> MFLIHFVHYKTILQKYTFKFKHIFLSIDKYNSLFFNISGILIWLNIIHINIILIKYSFFILINNFEYLIILIST;> MFRLTAASQKNLNSWYTKGTMRGGVPRIYYAWMRPGSFTRRRFEKMRNPFVDLETGTSLYFRDTRDSAEAIAHAADSKGIKGMDNAIDLYNEYRIVPDLYPEGFQWKHKLNTEYNQWRSNTWLTPDLIPKEHRGRFLCNFQLNIVAYDMRVVKFSPKDHRQWIYCVLYVGSGKGIAGWGRAVAPSTQEAKKEAIREAFSNIIAVDLEQEGPMYPVRVNADGVRVLLYPARRIVANFRVADILCAFGFQHAGCRINLKATNNPKSPTHTVEGVFEAVKALRSVSEIAASRGKVPHSLIYNIYPYLEEIRRRKGMMAMHPPGKDGLLMPDRVVDNRLPDHLKRGYYDDVYWKDFFAGSDEHLNEPRMGLRGDEMRRRLEEAQTSPAPTTAKDTRRRTLEDVLKRLGKTTRDLGSIPIVNPRVDVGLPTHIKRNYQLH;> MVFYSFVLVMKPRQRRFTSQALREIGVAVYSNGGLIRSITNEGIMRPYSRFRDADNTPLTYARYIILQLDMGEEEMGKVDKIIREHQDVLMALKLNNLERPVGIRSGNKELQAAYFPLDTFTRLEEEINWSPQTSADIYTQLEMNWKEFSRTRWSSFLRN;> MLRQSLLSLAKVYGAVPPLGAAQGHRLLHGKREREGSLFAVANDVKRDERLLRQQLNALLEEERMPMQARLQRNEAVSSHEAVPQTPLVDLPGVERRRDLPADPITRLFFQHKGDHALYYGTYDKPSVQDDDRVQIEKRVPRRREENLYTPIYDFCHRIREATEQRKRFVVVPSTIETRGCARVMHDHGLVAGFRDFHNDRAFAVELKYFQGDSTINVIEPCSYDGRTEFEWSPKMMRRLLNTHGIHNRLVVYICRTADNRIIDHIHAVKENIGGRGLMMVH;> MQKLLSPRTARHARLFRLAGKLADSGSPGVPKSDGERLVWVNSHVRRDKDISLSQEEERIRELMMPLEVGENSFAANGQATHGNLFYFREYPMYPGEYVPAEHNTLSSLRDELRLDLTAQSLKEAWMRVSGGVYFQSVDEYYASVDGLDAEQIGEVLAALFPELNCYEAQALVQRTLECISRPVSAASRQLSRTITAEAVGLDNAPGHYTNFLEWMGRLTETRAFKTEHALFEFSRRKFNRDDVRVMFENYRLMSKATLLADSADSYSHFYTVLKDFARKVAGEDSRHQIGVRIDEAEVDPETGIAVGRGCADGEKYHFTALLRENRDHNGIITVMGKPLSLVLDNKAWLMEMVLMPFDEANLDYRDFDAHIVSEGHAMPSIANEIAAFALRMAVANALVKLIPLTRIPLKKSGLLSVDRRRERGQFPGYLDGKKVKRRFAKR;> MVRRSHVVAYYWSRYRMPTQMPKFDGPAPVAAPQSMNSTKTNEFIDPIDDKFPMSIRGPLVRPDVPEDQYVDSWYICTSMTHHMGDYRPWSASAPPNAFRFRPFNEFDAKGREYVQYMREFARFDPRKSRGNGQKGFPFRDAYLTKMNEANQKTPPPTLETIMDRAVREHHQHARILSPLEVQRDVGRLEPIPSYAGKINADRSVFPFQWKTEDWYEYEVAKVRNRRFVFENTEEDGIRGSEVTYKIVLEGFWDHHVMKLAEDVCMFLKDVGRQIVEEKLVAVRRLLQGGAVDPELLAAFNCARAGPFGGLDEYDKEEVANFLRSDLRRLEEQCLSVINRCNVPVPGATNIYDPHTSWPHVEKLEPWVRMAEFWTSSSDTSFTELEMSTAHYEFRKFFRVIICKLPFQSTEFEKRMYDIRHWLHRQTSCEFHTIYRRNVIHDSAVFPTEHDPATPTTHEHHRMFSFALDWQSAPVNRLSTDTVHEGESWDAVAQRLGCSVGELKDANAERETIEAGVVINVPVTATRRLTSFGATPLVLPLKTTSAKDGERIRTWEEAAAILDCTVEELQQCNGHAALTYQKKESEAGEFDSSVTELVAPLSCWTSTSESEFSPVERVHANDTLVAIARRLQCSEEALRAVNDGITDVSGLDFVRVPPEARRPRRLVEPQLRPQAATDALLARTIAEEETFKLKSIPHLPQNAERFPHEYHTPTSRFPPTPSETPATQDWMAYTAKYLDKQFTISAEPAPVYNVNKLWPMQQIPGKVDQTPFEEDQTWLLHSIPVQQLEMHHHEKDLQDLPFINHEQFPRSLEWNAP;> MMRKSVTFLRRGKPRPRAGMFPDKYRRVPMLLKPQQGGQQYFNHFLIRSTNDRLTQQDVDNASGQAHSFISPQLPQMDWRNMSARSSEESIREEMRQLAENDVMQHQRVFNERMWYEKEEEHRMKARSCPEETSEHAISNDGAVPPPRVLGGDYFKTRFGYSLVKNSEMTQGPVDYSQLDMWGEMPRYTSDMVFLYLVSRRRNTYAVAYTYEGKRILNTYTAGNRGLKGGDRGFRSEGSTDNGHQVTSMYLNDLLPKLREMRASEGRPMGRGEKVELVVRVMGFYNGRQGAVRAVQDRANEFHVRYFEDITPFPLNGPKMPRGVFK;> MFCFSRGLWMRHIGQDVPKRHTHFVLESRLMYEKSFRDCWLHSVCRAISQLDEPLSKTVVGTHQKMLQRKVTCFQYNQYGLFKTPYYRLANVDRYHAVQGVAGTREWVPYVNVSYWTMNKMVRGGNLLVHRVHYTGWGTDSHLKKGGWEHRWNKVLQRNVLQYSRI;> MFVRSFCFLRKYGSKSKTPDLKTSFTKTTNFRKAEKISITTTDGEIVKGRGKIRRRTHSALKEAIGAMEHPAIWLWYPWRMNPEPPTPHMPQRRALKNVHGAVFNDLTPVQKKRQEQMLYGVNIPETRQMKFEEQHPLLAGALRKLEGQPKGFPFWYRKYPTRRHAYEYRFSIPVEMLDGYNDDVKKALSKGMMSIQEKQFAQEAMYMERYAEHDFDTTSPAVLAVKRALKCRVLRNHLLTNPHNNIIKTVLANTERKLNHALRRLRKVDFKKYWEIIRDHDVQDILQPPNLVTYRQGSYWKYDWNAGLAISTNLADVMDPRGLNGCVETGRSRSEVARDLGLSYTRPLHENEKKQLSHQAVYYERLAKFKMEQPEAARAMERERFVRKFSGMFVKMDIRSGAPDFPSTYRRLLGTKVVRWASKRHGPN;> MQVTETVLARAVIKRRSPQLWGAPGAPIIRMRGHHVVWKFQSYDLVVEHTHKRRNSDIRLLHYLGKHCPHPQKSLWSPDTPVAQDRHLFMLTTVDIDAFKYWFGVKRCRLSMKPWALLAKAGLLPPSLTQNSKIMPKPLFDKESLMRYYLANRKDEDVMAREKYLNYENSMVKTEEERAAERPVAPYL;> MLRRSLLAFPWWNFQTEHRQRCVLMYGGARTKNTHNANHRVFIKKYKRNAFPNRTRHHWAVSMTGVLSQRPRRMPWPYDLTSLIFNQPRQGSDKIGYVVGTSMLKTAVVATNHMVYYPKFNQRVSRTKRFFAHDEDLACVEGDLVHIKQCRKISKYKHYYVFSILEPNVEGRERLKLGLKAVPPPLFGYPVSRRIVKLNLTSTEGTQEKLAAAIQEHVQDAYRFSGPTPDQPRNRLADPVTFEDANNMIAPNAPAAAALDASDSPPLLDRGEYTEVEQDTRNKKGDDYWMNLQPKEKYDFKSFKKSPRPLEDQVDPRLIDGKYDIPTTASENLYFQ;> MNRTGGSIYAHALSQFAVCRQPWNEYIGLLTKQDSTPYHTEPQEKPAYRGRKQGREGWLFGQQVQLHYHRFPDEQLITNLSRWRTGETVGDIAMQQFRNAQPFDIEDKDPQGVQRPSPEVYMKLNYKNPATISRFLTRTGHMYPADILPLNPEAVVKLRVAKAQAIRIGLYPRFGNPFWFRSQKFRPKAYQENYDPTTYSTKRTVEHFAYNWVQTDRIRRYFRELEAVHTSGSASARGSGGGTTAEHKQQDQFYSPENQPISLHRNNISYMEDVGRSVKNPTVPGLMSTKGMKKKFHNLYSSTSTKRMGFSNPTLGIKKV;> MAFRNTFTTPGKFSTVSKNIVLLLIWRVKVFLRAEGFAHSLVMLPVSLYSKILLCDVKKKIVYFHCCTRKKSMLRRCPCVWPDGPTKSSVSIGTAFTLQKRFLKIAKSAFGFYLARRGQRKYPFLRRPHIKNTHSMNPSAPYFWSFMTAKSQMAFLPEENYITGDWTGKFFVSKRQVYTLQHATSGAKVRVKSFPSIFEFNSPSRWNIGKEMNTLTKPRMDLIDEQMLTKKQRLDYVRAGLLPK;> MLRRAYIQRRYPFNKRGPREHKSWKHHVLTEPPKPLQWRDPKVWTRDLSVMKSFDAPQWDLWQSRPRSEDMDEALQPFMDMPKSLKDRRYDIPWWANPFGAWYLQNILSLELLKLKSKTNAEKIATYRSYMRSLASGKDNTMSDDDVIRNIIKERWKTLEFGDRNAGYPCTFGDYIQFLNEWFKSLDEEGMQRLREHFDRRIRPLLAVMSPVDILWLEALTQNSPHNKEQLQRKIAFQTSLGTPEFFDMSKRLRYEINEDYKVRDELGPELFALWSKAPERWPPERLSKMYGLDFTLVRKILVWHHFKACYDACVEPDWSLPKRLFALEWIRDVRARKHGLFYGKMRFAEQKITFYSDRFLFRDLVNRREASYANVWEMDDPYRFLQTEQDYEDYWGDNYDVYRRMFPEMIGRTGEPVQQYGQMPIWAGPHRQHANKSEHNWMFAEIGVNVGHEALKKLELDPTNEKRRRFVIRQPDGTLRSAKMSEMRAWYWKEEWADFRFWAPQMEWGIENTPSQEQYQEHVPDTTDADFRKQRRIQSRPVKWFYESHYTRTGSFAGFQPLRFMQRRTEREVRWPDVINAAVQIQKRKPAAYIFKAIPEL;> MRQCVVRRYKMPKNMGVAPRFDTWNEKYEPWEHMKRMGRLVGTGFYIPPEWYNHFRMFPPINHNFQQEKTLNPHNASEPTQDDTSTLSPERVALRDELARKSRLVASEGMRYYNIFWVRKPLDTMEKEYYELKRRGVDHGEAIRKVLQGFYSGLAVKKRVAAIQAEEAKLTGRFITMREATVVLGVLAKLHKEQLTPHQVSLLAKEQGETTQSGAKLTAIVSRTQPHVNKEASSPATSEAVGSSTEESLSADALASMLSEDGEQSAVGTRYQVEVKETANDSVRQLREKAEDQTGFPDWYTGESPTYSGTS;> MMRSSSFCRRQIRPYYNLPSKSEHGRKMTGFLTPYRHWMWKQNELWRNVHEAQFEHLRRVYKRQWLESFRVNADEYIYKYNITKAAQLAQWECEMKEQEKKRIEARQMMDGRQALKKKHLDLLREFHERQFFFWYERASERLQNMNLINYVPHAQLREHIDKELDKYVAGKNEPYPLNFVGQMPFLEDGDGNIVEVPESLLSNHMAEHPDSTAKPHEPHTSSSISEAAAFEERMLRAMVSAKEEDLKEWLGDDSRALSETIDDISREEEEREADIRVARSMEETDAEREVSRRAYIERGKTGSRSIFRPPTVSEGAGGTPSAPAGDANTPMRRRKKGKLDRVHALQAHQDELLAKLSSQGLKEGVDASSVPERGKIVQSRGRIRDKAVIPTHEVLMQKPELAAGSTPGARIQTKDMVDKMYHRGKYKKSGSGDKSDGEDL;> MRSKTLKKSLAAMYMRPPVTCYTDACEAPVAMWDGAIPLKETRKLKNGVPVRTVSRTYSHPPQLTPTQLSFNDINSMYCVGNDELIQFFPEGLGGRVFQTMPPGHPRGFLYRKETHLLNLFVDKVQHWHTKRSVLSSLTNGRTGFIVDGPTGCGKSALMCQVVHFARSRNIVTLYVPDAKVWTHGEWCWPSTILPGFFDAPDAARSFLKYFAVANRATLTSWKLRCTPKDLPTEQGERQPQNLYELCEWGHRAVAPASIDRQSVCVKFLMDELSEEKKLPVVIVVDGWNLFSHETHFRYPHPDFLRGLASFNESSTDIDLYPQELPRIPASRLSFVRGLNKMILSGDDPNKFFITCTTRDFKPFDGISGFPNVETDRFANSLDEYAPYDPEKDSHFHPIQIGNFDEYEYRSFLRFLINSGELAGLGWGPLWHASSDFERKLYKIGFLSGRNPQGVVDHYHQELVWRYDYQRTRQKQYLLKRRMEGMSRGASSGAVGVR;> MVLRRWFPLLGVHRVGYTHPSTLPVPCAQRWDLRLARARIFQEYIEEKAPGAWQLEDERSMSPEFKTFTGYPMRDMRPGYGQNLPDYIMKKRLPNNTHYELFARRDIPNEDNAMYGKYLYDMTVHGTSLPSTYRMHKDINKAQRNDRKLSGNRFKVLCSSGAKNPPSGWEPIPDATEEEED;> MLRCARVALRADPLNGGSSMTLGSKGSKLSPEPHRRRMPWTAAKEYVPGVVLNARDKMVLDGVQLLDIESIDRASQLDPLEVLRAVVATREYNISTGKNIFQLASQATYNGRGQRFYRKEWQEGTYDKYVTLSAIDFDRDGNKGTAYGYITFHGETTTRPVQVDFADVPGWYMDFVEERAVPFTGIVPPPPSIGTDVPVDPHSYRLKAYPYYDAPNPPEFVERLLKDRGVLPDTPTETADVDKDPTTSDGSVHYDGK;> MRRWHRSLNPALFGERGSGHYFSTTRARLQLQAQDRIICGTHGAGIVAHQTAVNSSDNPMLSSVTTAAPAADLSRTKPHEGTGTSERDPYIRTLHNQRSAAPESSVSQSHTVNAPTVDECEMLAERWGTMNYWHNDTFPRLVVFLKKLLVPDVSPLSPTAESLLSMFEKVVIPKLTSDEEDRRKLVSLWSETTLQAEAAVTKFLFQRGSFESMLHRIITDALEKMSTLALGGQEGNLALEALKRQTLFKRNDYIQKRLIDVVSNSAYLGYGDSVWQVFFAAVEANEENLLSDRATTDAIRAAWEGVMREDVVRLPDVTGVVALYLTLVCIRESGRLVPEELKELSSGLEDGVRPGVRKLQQYPLIFLHPTVKRRFVVKAVAEILHNSSSNAFSNMLRENGLHDTAREVALCEAMNRNKELAEGDVGDAVGRFVSKGEVKTLLSSLVSGTDAVVRDAVAGIFGIGTTITIDWDAVMQNVDWSNNWQRLATALLSNSAVLSAIVKLVKNAIGAKGMSKHLFTDEYADQLQLILDAREERAASRKQRIENIAQELSSFERVDLSCDLLRKLGVDMTELDTAAAATRNMNVVQRPCIEDGLLSLVLEAVTKRHPNWVKAGVIQTTLKDPFDALRWMMHIFIRLSYVPHAGAATIARLSRRRIGPIGLEPHQFNVPAELGFVEQYDNLQYKRYDWQGWYQRMLDVHNRNVSLRCRICDLQRLDGNGVQFVDMQTERRLRILAQHRVGMGVLKLDADKYEDQADNVTFGTTKLSELLADARKAQLGEEYWPSVELKVRKPSGQSKAHYSLIDNERIEKRSRELYEKYRDAKKRSLFVTPMETWLEVKGMQVRKSVDNADEDGYTLDALQDMMDGDDGDKV;> MRAGCVACSRIPKLGIAALGSTTTSMQATCQETQELRCATTQMAPAVIFPLPPPLRGSYIDRKPTAASFNEHHATASFRHHMIASADVSHRPRHFYFASGTRNDTGTRSVKEGERKQLKQQTNVEVDSVAYGDQLDELSARWAAKFYGQVTFGPRNYPYPSSRWLARRFQMKKHRIIKRFRFRRYKLAAVANLPFAKMIRVGMLPELKSSKTKRGDVVDPTLSGQLVSAVKNTGEKRKGQRTRPKSKYQV;> MLKRTLTVLDQTYGPHKSYKYTYMPDPRKLAPIETTQRSEIVPQSIRPPTSYVPNHETFLERADIHRLRPTSDFKASFKDWNDLFTCDKRQLRVRGIPRMTRDAIRTAVQAFQNGNPPERFDTKEEWLYYKQFKTVDYSYRVIPELPEKYRPHQSGIDQAPLPDYREINKMPQWAECEERRQSKKTV;> MIRRRVCDGARLAPNIRATFSAVRYQSGLHTFIRDSKPSNFSSVRRSENANGDATASPGATAGENPASSGDWASHMQRELFGEVD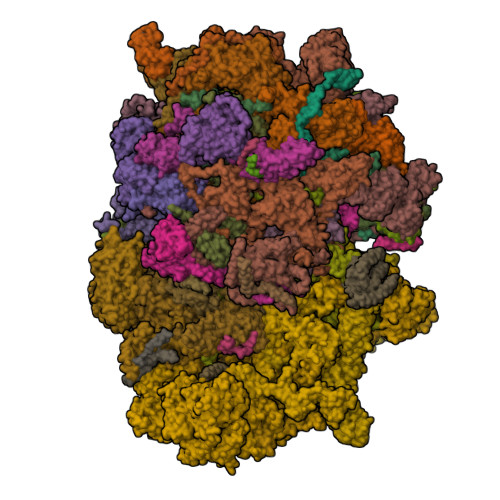PLGGQAHKDYYRDVTRGYSPQYAPRNFANGGAVAYPHIQSPYEYEEAAHRRVWLDHDVDRMREEFTQHRASLRSLASAQEREELLRSRAAEYQVANTVHESESVHPIQQLYNSGGTSRSALKQQAVADRYSIAEQHSPLPLTTGVDRDALDEAQRTKDRILNDSFTAENLLITHGLREKEKHDFTILQRTVRIPFQGYDMDRFLAQQKGTPYGAQQLPPNVVPSSMEEAQRTLRGSSATATPLVDAVAQKVYARNTVVDRPAIGEQLTEQIINIMRASRTTAEQQREEERAQRFGLGRQGALVQDGGPDQRTLKKHTNDERIVDAMLFQQNAYRKTPTDEHWNPYIRRSTENGVGHLLQNKFDIMRREDRLSKGEQDLTERNTIHYGVPIQQIVDEFVFRHRNARGERPLDYFKPFPNFRALRLNRMYRDVEGFSLMKQRPEFLEWELFTRYRQHHQQRRRLALLHGLEPVANETAQERDTRRHRLDEICERTPFDEREMRVNDDEMRVSVETLRSWFGVYMLPSPTVVNAVLGGSASVNLHLYHLADEMGTADTREHVLSSRYLNRLLLLESYQNRVGRGFMNHVVGRAPEPVVPHEQPQEVLRHFSAEERAMYEQHVKEQTSRQLGEWERAMKRRRWLTDHQQYGHVVSHGLETSVVDLSHTETGAVLTVSTKAYEQEIEAVRMKTNATIKVDGMVYNLLPNSERRVVPLTVQLDSGEKIDMTSEDFDRCELEAFPRNLNHALNYGIANYAYNRGNYVETQDSIWEEQTASGQEGWSPATHADGLREGLPVRARRPIFSSSAEQRIAGGPQRAVIIQYHHQPFFNPEPRLVKVAFQCDGTIMEVPISDVMIWQRRYHGPERTVGDESRRYNPAAMRRYVDVTDPFNEKTSNTEHFLDKYEPKRNADTVADKYRTTKQITEIDKWTRYDSARADNYRPLSISHRRDYIRMGYIPRYTPWEWIAIQEADQPLIAEQIRQDNIGTSYFFSLNRYWRYKASPHGYIRHFENEVRDLLQYVDGVTPWKQAQKIRTYWEVRSHHPMPQFNRPEVAMHRNTVGLLPAHMWETDKKTGKVKSVKDSVRDYQTKTPYPKWVQL;> MFRVRRLAGFIQCSPCGKMGPLKQQTRRYTPIWKSDPAVDNVAPLRDEDERRALWAEVGPISDVGSAVTAWIRFGNDPVLHTAVPTMLGGKFRNQQREKESLLPNSSSPFAYVEDYMGTNLVFGSPVHAKESAAVWATYFERRYASRLRLSRRTVANYVGLINSPEVFDDESDRPETRWSQDTFFRECAYLSEKFLKEKVSNMQQFEAALKRASPEAYLAFFDAFQQQTQTQIPLPSPSVWHYEGERRKQWAEKFISISHKAQAFFKDVLSEDVKKYQEVPGKLLQKVKPVLADVGKILVKRHERWLKGRVWTSLTEEEREAYCMKEVKRQQMQVEDGEFDPMMEDDVDDTELEEWQREHDAIMKLMNSPIDGLHFTTLELWLHTMRCEELETEHIYTSARVRAIQVAARKKLYDTTSYEEVIQAVVESIARGTLDLGAGVLRPHFNEVWCQLNYAKFGSSTITQHTTTSRRQLLFFHAGSLKDIAATATLYYATKPLSNSLDYASPYKYRRSLITLCSNYGVETAYTTQRPLLRSAANLARAEDLIHAVVTAAAQPFGERRRAATRDLHMEFQRLAVPVERVIVANPVSALLESGADPDEKPVEGEKVNMWPLGAKRVVLYKWSAPNVEKLKAMESDAASAVSGSSLTAKRLREIQELKRRGFLEVSLWRRVTAQERKQRNEIVEAKKKQVEEVVRTVPSLAHLHQYATSLYSRIEERVAFPTETSTVTETTNMKEETNKPLEDSEWEFAVLLDDRVLLNKEESVELYLPYRDANGELLAQGEYRALVRAFDLEANPNLHPAYCSVGYSESFQVFDALPQLIAQFFRVKDATAEAAGVTHIPAADFTPFCAFLRDAGLDVPLRCEFEAGQAVTTDGDVYMDYFLQLLRGEAFHQSHAQAGLTEAQRAIEPLCRAHWVVHHPGADESEWATARRSVLDHAMQHEREWWFPNEMLDVKDVVTGSTNGLTPQMYPAAVRYGVELCTVLTAEGKFVDERGSGLSARCVVNGTGAAESVVFDTANCNGTNTTSVEDALRVAHGALRSAQDRHNTLAAFRLGPLSKQSQVLLFCGVNAYEFGGKYARTYAYAFEKAKKELEATAASGFMAPSLSHEDTERLSDQPTTSPSVDRFASTTHPEQRKAQFVPRVGPGSTPLEDPAADQKSEWS;> MLRCTVVGHHRSGKARAFVFRDPSLRMMRAGSGYQQLRRMGMPMQVGMGWRKVDSFHANTQYQHAWPLLSHDDLGNSDQSNNTKNIMYSMYMPKRNKGTAPWFRGADTYSVKYCEQGRYEYQRYLMINRFPSEYKKHFLSFLSNIRMSSGSATIPQEALHWLLRMIVDNFNPQHVHYIAAMKTLQSAGELDMARDVWKIMERQQTWPCTATICAYLDVCVEAGEKTWAMEAWNRYCTELKFLEPGEVDPKPISRVPFSLTREELLYLPKWKKHFDHDPNLDVMDLNRFNRTREVYLRMAQVMLAGGERNAFQHFFTKLEEAMLNKPTPVPEPPNPHLVRRPRWAPYEHCKSVHHSPWRLQNNGRALALGPPVTIEDEMQSRFFSNDQFLVHSVKEVLRIVLQEHKRAHPTECTRCKTEAFFYKTKDADETLKFCDDLIERLFASLGVRLSNLNTSSLLSTILEVFRVVGKESGAALLQRANEFLERKASLGDAEGSRENLTASNYLQVLSGFADESAFVYNTKKDGTCQYKTGFDPRTTMRHLADVVQEIAGNPHVTWAADMHLQVVETMVGCGTMKANDYFVRNVLRQFSWDSRFLEALYVEYRRQDDVDMWAELTKRALVWTARYNAPASERLRRLIEDDYDTIRVQTRTFRELAVFQFRDVEERRHSRDVVNELPNPWYDYVAHALPFPDRDAGYPDEYGDLGQWRAPGGPGSPVRGPGYYAPPMEGEHQRGYTAEWRDLRNPMRPPEFPTPWERKYRQYARGQHPSYDMVYAGPMPEIFPMRRDFRKPTRWDFHDIEKQGKYRTSGPY;> MRRCSFASTCRYRSADDVPLGLGSAYVWTCRNITSRGQFNPIHNFSYAMERGVRARDVKAFEKLITNPGPLRVAYTPDYLDWLHRCYKAKGTYMDARAVAEKKFNGNIVSSELSAAVNRREGKRGDTRGDTVDNDHHNLPGAPPPGMFLRPAHSFRRLAGELKRRRAQSILDEVARAQGMLDLFERQPHFPAIHIDRCSRFHLVELFKEMVLERSLDSNMIWEKALLYRAILSERKPSYPTSFHYIFTAVEDTVFAPTISTPMEMAGSGGEGHDRSSHPLAAKCPTLEAYYYYVYLVKKYYIDNAVEAHVVLRCHREPNAADLLFSNPPPKDDTEIMKAVELLRNADIQRGVAAAAAVSDPTLPPGGEGSVIGNSDNKKNSEKTSEGSRGRPARPPVLPGAYPPIDMLWRCEENLPLLKVLLFGEFNLIVSENPFVKFPSAHGFLTRPYSTDSSRTLADGMSLANVMAEKRGHLLPSLPRNTATSIDARAQDIRRLQQKHHRDDIVSFQKLLRSTHAEDSPSAFSSYSDWSYFNPRAVRAEERDRLTRKAVEALKLYDSATNDIYRHSFEDVQACHTQRVTERDRTMPPYLPTLPHFVAIIKKDPHISFLLHIGLPDRNSSEEGSAKHKELEKRIYYLARALYHTALEYHNETVRRVNRQKVNVAASLLDNFVEQEWTTILRDKHDVTDVTKTLNDTQNDKKQLARRLGRYMLFANRSLDDTGFPTDARADDYTRWMAPPSVGKVSL;> MSVSGVFSKGRGIGHEATTSILRYIPRARVPWQPSRFGRENLTAADMARLWSRGRYRDGPGNYNSGYCTERTHVLEENTVSIIPRRELEKYMPDITIGPKALVTPVSLMNARNGHRVTHDLLHSYDPHIGRLGKPAVVDHDNITVEDPNRVGLNAATLDCRGRIYRWLRRGPFFQVDNYFRRSVKLNRDGTLPTDFVHEAPLMRKIIRLAHRGHLKAACEEYRRVTTVPPVEVYRALTACCVPGAKLADAVSIFEDGDSKLFYVSRDGEVLHNLMRCAIAARHRARIMWVYNVMRGRFYENVVVRAEVDLIWRYRIAMIALEYLLDHECAEEAAAIYSYLVEEELLRCDVHVRVGLHMREAIAAGKPITLNNDVMNATSLVRDATAVAPEVARELQRRHAQTLQNNAVEAVGAENVREGSAPWSILGPLTAIGPTAEDTMVWLQQHYGDVDVMSIMRWARFRKGKDLMAKDRPQYLARAAAWIELLSKRNREMEEVPLTYMRKSKPLVLDTNSNVRVAWQTPLMRSGGPPRLLAREEGYVFHHSNSSRFVEETYRHPGESLQSRYLALQPLHTEVSAKEDFQRLYYQAQKHHKQQERLLPVSTAAIPSRIVHHSVMSALHGVSGKGEPANRSLFTGNKSNDSHSNTGVASGTSACTDGAGSATPEF;> MFRRAIPLLSANIPRSVWDPAQHNPNWSDSYGHDITNRRAWPARKWTVGLEPCTPREWLQFSHRNLAYAYNGALRACHSLPSMLLLYKEMKQRGVKVDVDTMNVLLTRAARHEHIQVDDVFLLFDELVALGARPDLAAAETLHTVLSHSASMPEEWREARRLQLVELYNNLAMEEVERLAPHRADRLLKEQMKRFRGNLQQLGSGLRPTVYCRYLHTTHTAAVLLEEVHNFLWELVPNDHPAMEIPALQLRVPFVASVLRRPSVNPGVSLASVSRAEFGDTDVCAVFLAAAERMVDADFDDQRPVSERRLFLSLLTMISYSGVLYTSDLMAQLMEMVKYSNNDETRDSDAQRVLRYALRGSSAAQDSASRTLWHSVEKVADCRVVGRYIGARNPWNPIRVCFDEQGVFKAYPISTTTTTREVSPPEGNGAVTQEQRASCVEGRTLEALNMRWDDVRRLIECTGVLVTPPSERCPQQQKMEVFTGMAVYLRTVATGRRYEGGEDVLSDGAVATSSCEQRRRGTLFAEGYDFDVWVRLFSLVQEVRHDMEKFMADHTLQCVEPEFECWEALLVTLRCALDFCVVQMQGGGARGTEREVVERLFRDVVALREELIEESRTRFGGRMRVLWLQEA;> MLSQNVAKTTVPSYYMIRTNLPHRKPQNQWEGVYYYSGITKRQRHLILLHRKREREAHMRSFNISRASVLQRLEQLSGDRKQESLPPHVRLDLAVRLAQHGLYQQATPIVDELHHQKALHAGHYALLINALACPRLGQRILHCDAQCDPALTYKLLGDENGEERAQEAYRWFDLALTSLAVDCGGRTQPSHFVPYLPQGTAAASHITNALMRTLLTCGYTHVAAIPDSVYDRMGSMGISPTISTYELVMLALSLQGNMVEAESILSFLRSHHSEHITVESFNALLLGHREARQFDCCDAIWQELVDRRWPRASPLTAELYLRSIMDHANTPTSEPLQSFANINVVEKKKVPLVLAQMDELGVPRTHLSRVLMDEVEDSLRKFQTYRSRFYEWGRAVKQFDFIEFRRRNGWLYDLHLMKCTTKQVGPLRDFNDPDAVQGAVATAEIPAFFNERPAWERPPLEETLYVTTNKERYDDVRGGDIYYDDTRGLHDRSPTWMNEVPETRYDRLYGVNHPDIAKIGIRRHLNVEYVNRKEVVERDAALMKKTLSSGRRLRHRVESSRTHRNAGSLSGISSTAGGGSR;> MRKFCHFMANCWNSARSHATYGAVPLTHSQVTSVYATDGGKVDELGLLELVEERIFSWKLNKWEMRIPPNLPNDQKELIRQEQENLKQILSEWRKCFGALNADILQISSLTGVPKDVVREKNRTWLQEEVAKLRWMGEVNKAALLRDAFMRLEAFGSRDFMFMERLCCIYGLARQGTFDEAFTNYITEDPVTNDIFVDERNPFKELVAHIVRNYSQIDIIYDFLGFNYSEGYRSSLRRYMEYLQCKTAENVRASGRLVTGDKGEHNILFDYCVSRESLVSGDSCQGIIDFLYINGNDVTLIIIASDNPWLRNRQLPHRRQMEGIARRVCFVLGIPPSEVRIRNLLLPPTYLDKGSIVRLNDIVFRLSNEQSNLLIPWLTNYNKELDPKDVDYTALAKTTNEEEWLTL;> MFRSTRPRSVGYTPVNPDTSPMVAYSQYHWHYNLPQGMERPHSVNRTFAAPFQSNHSLVNKYRGVWIEFDMHPAFSVALEPQLRKLPRGRTLPKTPAEEVIADYTALAPLVDDEKTRDLWLAKVFQHCAFQRCGGAMELWERYCHQRFTAEGATAKPPLSLVKSVLFYCNKTDNSGWRALFDRCLKDGWNYTPLFDTAQWSFMLKSIGRMGDEDGVRAVLEEMLDVQADLDRVEARSVVIALNAVTNADVYEFVKKYLFNFGERKVKFLRTTYSDLRGHGAGKLRIPLKENDNMYYHVCWHSSIRSPRQFSPRQLYFDYTPSTLGSSSHNPNAKIDDIVKDKIEKWKAEGLLPEDYVHEDRVYDRSAAFKNVARQEKWKKMPKILKSKRMGYTGDP;> MSFRYTNNLIGALKHRLLLESSYREIASRKFIGNCRGVEVVCSGYGTVLAVQLTDKAVWESFYRKGGRPTVSGGGDVSGDAETGTQGSATTTGATGSLDLDKLAESIKTALWDATRKIRSAKEAALHRSLSHNTRMRASADLKHWYEEDANTLRPLAFEALKHEAATPWMQLVQHGKKEEAAALLKEFEQKGDAAEATPTRVKDDRVKGTRTELSNREQPPLASTLKAEDSNPATIPIGSVHPLFTPALVQIEEAGGGSVSNEAVCRAQLWELSRDEQLFWERVELIRKGQVASIGSSHKRGYADEAAFAKDDTEEKVQLRFTQ;> MRCSCAFLDKSVFAAKRRVIVPIHPTPNFPAHFIKSAFTTDPLKEKQKARFSSGGEAMREVQDIPKNLEGERSRRDLASRGDTEFQALVEFIEGASYDQLISGRRFKKVYDVLSENDDMFIWLCHTAMSVLNPGDMRSRLIYNHLRILAESVASGEMTQRTAFRFFESAVRSPAYREIAKRQLEGGAATRLAGISAAADVMRRMGLTRRPMSSYFELYQRIVERSEAMTPWGFPPLFQFEERLSLEPRLKFFSRASQQSLERRRRGHVMTPHTTLHGRRIFWIPPTWNRAGRFLGPHVTLYPGMTPD;> MRRFCTARVSSYVKRAPLLLPRGGRRWRSGAGTTADGGGEKEYIADSFESTAGSNAYAAMELAAEARREIHELWLSAETALEREKRVQQVAALIEKYKLDPSTPREADVSRGLGDAFDRLLLLCLPLGKTDAKGTDNLERLMHLAGRNGRELSVRTIQHLFARTDSFAEALAVFYTMRRCHVAMNMEAYYSMLYSLQRLEEEGWGQHFRNEYEENGAPSEQAMDFIVKGISNALLPENKPWLGRVMFQDRNVPDRRYDTRDFDELDTAWTQRYKSGTPAGAH;> MLHGTPVRRASLRYRRPYWMMFLKGVDNWKIYTVIQQPDHQRTEMLYQAWLGGLDRPYTRPKCMANQPLWLSKKRHMLRKERLDGPETPLEKYVLEWHKKFHSFQGTERPTPDDLHTALDLVERPLDLSYALQLLGQCRNLNNIRFAKETFLVFLEACLRVGRRDCAEYALEHAEPLGFWFIDEDHRRYLQGEQTWYKLSPLDNLYYPVEENAKLNEGRKPITRLSPATESPGSGTAISDGEPSTDVEGETTVDDEIAQLEAELAALEREGGGK;> MFSESLCILSRRFRYNTKFPALVSYNKLPWEVVNHETPQFHMHVAPHYEQLLTLAASSPVPHIIGSKHIDVPREHRLRLLPGMLYLLDGDTLPGEFTINRVLDPTALQYYGRLSSQIVTVEAVRMLVPDDLRLLCNCITFKGPLHLPVAPYASLASLRGASQGGTTGSETGSNCFTLYHFVRPNRPPKELQLEKYYIHAPCVAPLSEFASNSDERGNWRPRLQAPKRTRRATPLPAYRPPQSYLMGLAERLAVVPGGCFGRRSLMWGHWF;> MLVSYLRLQADRRTRHHMMVDGQINPREWFNWHPKEYQPWYFDRHKFLYEQRQYAQFHHLLCHQVYLKDMLHLMRYPEPYTHIIDCRTSTQKMHRWVPHSLWLPRDEVEYALQLSADEFLDMYGFRKPDKSDDVILLSHNGIYSEQAGWEWKKQFFQHVYNYRGGTNELFGESYSDMNVSDVLSPWKGPFPQSGVFVDKWSKRKVLTRTGPFDRQYEMQDFALPDLELEKARHPEEGPRQNMPFGLQ;> MRRGALSLLKAGLLGHYQQEAFEARKRFEESTTYPGPIRAATPGDTRFYSGSLESILHDTDRHYWRAVTDDPRVQHLIPLRIRFKIFTWVTSGWEQRMQVVQIMAPKDSTIAQVKDLVIVENQSPYLCVSSFHLAIDGKELDPQKTLGEYGITEQSQIDAIEQNDHLLHRDDERPRDWTVDEITAEDVKRSPYKEMEMQPLQNLAPRYEARPKGYFGRTYYSGMKQSS;> MRRVRDGLFLSHPSSALQCSVAVVSTGEFDHPPFQFRQRHTFNTTPLHDANRFGGRTAYLREIGPVNIKKQGRRFKKDPRTVQFNVDVWCAQQTLRKRWKQRDWEVIEIPFRLVPREQQRVIPELYTDIPQMTDPARNDFSNIRNKVYDREELQGVLFPAAGAMLYPPLQRVDKQAMTLDKYL;> MLRFTHRALTATPERFSVLGTTHPKPKRTGFGRNNKMRSKPSDNVAWYDKGPVEWLPRPVRLTYDHLDQLQQWTMRATLDGRTEEFNRIRDLHREWSQHPLMPVLGDVEPKFPLNLFKQNHRAKKRFLVRWHKANTPANWLWMPRGPTVVTPLHRTNPTQYPENWKQMVQRKSGTGTPS;> MFHRAFVSSSDLTGCTIALSSVCTQKRYWAKPKKRPKVGQGFHEKAQKWREEYLLDRHRALADSLRAYVEFSTSKRVEPWDARFKPFDRIEKDGVYVLMRYMMEEKLQLCNYHHRPVKRLFCNIGLMGPQITTKARWKPYRFATNPAGTSKAERMYQRDKTVYTHGHND;> MLRSTLTSLNTFLTSSVATPPISVIRTGPKWWAHPERMVRQKLMYFTLGVDQLPLRRTAVIQRDLQRFHMCKPPPRVGDSTGYKRSRAAQLNTWYRRIQYQEYHMQHLFTRHVWGLLRVYPGNTTKIQGKADDGYVGYDSVPFHRYNRAPLPFPARELYERRK;> MLRRSILFRMKYADLELTTRGEFPHGMKEPAFVKKLDQNIPWYFSTYRSMYHWPITGDNWSDLNEAEKHHDLHMFYTLAWWKLGEGIFGVDEDS;> MFFRFHSTTLQTCLTSGVARSSVAVAVPLRAGCTRREMSSGGDGVLEGAMHKPGESGLQAGSSTTIAGKETWSQFSTKMRYGRRRIRVIDVAAKMSYEYQMLRKMCKRRPAMRQWAVRDDFCDMNPGVVIMSPSMQAAFMKVFRMKEKGLIRQCLRDIVPVIEYRNREEPARLPTNPADMIPEGEPDTLNQKKRELFERREKGENFADLRLHDKRSQAKLRFRIRQRLLKFQRQLAVANAIASRSVLYSTNDAIGYFLFRGAAMYAGMHRVFFELSKQLPHFVPKTMLDFGAGTGTAILVAKEVYDPGSLAYPLYRSLRQTMQGNDSSRTHQLSELRYDLKRLQRNNEEKKKVRFMAVAALLERGEVDPADLPEDLKREIAEVATAAATAKKDRLVREAHARYRDVVDGTEWESGDPLGEVRASTEDPEDVIDGEQGDGGDDGEAAKGRPKTWWEKLIDVENETARTRAARRLRPLQEVTAVEPSPGMMEIGTMVLHDDVPNVTWKRYLLPEDEAIQHDLVVAAYSLSEIATSENRRRIVQQLWKMTKGVLVFVEFANLNNFNILMEARDWILEEKDVGLWDWQPTIVAPCPHEHRCPLRHCKTGVKRKRMRICSTEAHYRSTFVEVWARHMPLKVGIEPISYLILARNELVPERAERRREQLKKAEEMKRRERDVKQQQLHEASLAVKDVVFERLSDEALHRVQSSVPQPLTDIDEVREASTSATSTSLLKDLKDGATSTGEIGHMPTDVPRLVKTGNTRHNRLIFPLQFPPATHKFNRAFVDAGYQRQRAITPAEMLVVRQEVEQLQQRVMRAAPKYLRVVRDPRCHGKVQADFCTPEGDLVSGRVYRRFYGDRNRVSAHSTMRWQHIGGWKLLKRIRRGSLFPHNVPLYAVTKHAQIDFPNTLLDTKHSTVEQTAMQYNDPMSLVEMPDDGLTREELKQKRRLQRDVELQKKVEEKLEDIFGVNAKDWKTDDLGGGRLDARREISEQQWADAVRRAKIRTVQHTKNALPFAAKKRAAQRALQVRRRNVRLEMSGNRRR;> MLTPTRRLPKALSPYAQALRHVALRGATAFGPGAKEMELDMLRKGTLPADYRPPVQGRWDDTIERWAYAWQFPAEEEQDDITKSVERNASGMQALLEIGNKLLRSPPSPEPLSGKASKLYPPVGDMSSGNTALLPPNPTYDVLEQDVSELMAEDAVVVTSQPRLRAEELSAKYNVPMAYIDDSSEASNASKSLALVMEDVGLEFTEDGLTVVISALSRQGYGTIGRAIFDFASAMGLGPSAEMYRALMKYASRRGDVNESMALIEEMKGNGITPRIGNWHELMYTFYKAKDYPAVSQIVDNMKMYANIEPNEVTFVLQLKALAKDNSQLNSLPEAIQLFDQMENVYGFIASRPHYDAMMFHLSQSPRPEMRLRCEELAHKMELMGIVWNANTYLNLIRSAQVVGDVAAVEKYLSRMREEGIPASIGHLTWAVQAHVQSMIRIDYDALKEKDESPLPTWLEHLETCFGIYELVVRRGWVMQLPFVNALLRLTCQATILSMERTPDEAETIGRFEEQANKIWNHTFDEWQLQKDVYSYECYIALLAHQQRIDEAEKLFQEMILKKDLSPSRRTYHCMIFMHLSSGEEGGTARALRYLEAMERAGIQVRPSLLKKIVRVNNAAGYKRDMKRRARRIMQAREEYLARKEEGVSFGEGGKEGASNQRADVDAEGNSILEPLAVSPTSTLAWWEKWKRETVSKHELFTEEGADGTPKGETFEEKNEALRMMGITSSFQTKDLVPQPDRQKLLPLIRREEGEIAGSLWAMDGGELSYPKDGGGPQGWGVRLWRERQLVKREYQKVLDGYRPVPQLSTLGNSVRTAGDQLDIERSGAQTPGELSDYRNFPDNRFDGGQLKPESEAAPAVPFSAELVWQGEANDKLSPYKSDEEIALENDNTFFSSLSKETEGKLSIAVKAMQNKEENSVDVRGKGVTRRSKFDYLEKWRDMYRHGTLEVPEGPTLNFGRTPDDHKETMAALVRGWYQRNRKEPASEEELKRWRVDEQRSSETSASRAALKKRKQVRSRHRNK;> MLRGWHPNSSAMQVGMRHITIGGRHSRGGFRQPLGKHPQVKQGTVEGVPRRIPGTTKVTYTNKKGRTFSFSVPVSELTHPQVTLESAAGTWREMDTSFCELGDIEDDMPSPVDECLRGGSSLDKRLIQEVRERFVSFCREYVLMDTSGMKSTILSTELNAGPDYEHYDRRLRRKRHWLAIRHRFEDVRYVIWPDVVEETARGDSAQADVSLTNPSLTAGEMLEALLWLDAASTFCVRKVHPSDLGDKSEFLPLDLQREVEVVACHARRDLDFFDPSATSLEQFTACAALCVNHRVPFSLFFPAQDVCGDASVSTGQCIVANAPSPHTALGAVRIMALISEGSGSDIGKTIMFSDAFGAVTRFGILRGLSRVMSVEAFGCKDALENVNESELCIILHFCAEVREQNAAFFRRYEASEEDSDPQQVSFLAKYQQLSQIALARCKRLLYHPDSPRAQVMSEDGYIPLVELQRHAEGTNKAALIHYNLGIRSAQGMRRVALGAQSSARLAELVSRLEEASARVSGNTLVNDLVHHLSHKAAAGKMSLTLREVNTLLPLLSRMRRESPNGALDARFDRVFNAIDTAIGAAMRHNCTLDELLDLAEGLAACEMVPSALKQVEMVLIRSVMMHECSPMHLRRMLQAMFTLMRTSVPQVLLQSVASRVADYIKEASHMDSSSSNGGGDEKVKNHEECEQLLELLVVLGKCGYGALPGLVTIYWEAQLIDSMQLNPRLRCSYASLLASAAFALKKHDKRAWEGLADESHRLFMEYTRCNKENDIGRFAECVTGLAVLTQIKDNTNSSDVAFLKEYLSATSLELKSCEVIRVQELTDLLGRTLEWSEALGVVAPDVVIQLEKALFVMLENVSHTAPGVGIPDELVTAACCLVDMSSASLELRKAAAGVVGGAIVHAEEALETLRSGAPTQVRPGHSFDVAALASAERENVYKNSILQYCAALQRSGMSTHVEELWS;> MRIATSPTRRGKNSSVLPLLRRFSWGNGMCSPYYTEHRRQSTLTSSALSSPANHNQQVVYRSIRDCRERAFHLIQELVSSPIPGCGLSYSTNGSFGGPSLTANAVSGVASLLELYDKAYYFLHLLHRTILVPRNVVRDTDDFTEFLLRCFRRPSDSLLKGDEELQLSDAAIVDGFVEWMETSLMSAGQFVSFVEVLQLVGSYVRYHKGVRWGARPSEEEWYRCGYRLHPWHDTYCPSSRAEQMPYVHLLQWLMRAKPTKLEEKIDNKEGAHGASSLFSTAAKESAMRAWYATEEFSPPSWHTVVGNSNRLGFTALDCGCHSGYMTELLLKAGAQEVLGVDVSPHHLGNAEATLSEHLRERRSSSHSRKTVQFVRCDILPDLSDEARQTKTPPLGPEGSTNSAAAENRRRLARCHHMPSDSDGLKTETEVTGPFDLLLFHPPLPLLFPTWPLFHDLYESVDQLAYDAGRRHPHCRLSVLNEFLQRLLGSSNGEENNSERRRNAHQQLKHQRRLVAPLIKDNGYVAFILPRNFDTRAILQRMSTSSAGKNCTSCGSDGLAPLVPLSDVVTMTLEGSYTLVLKRSHSLSSLLNRMDYIQKSISAFIRAFVSPQHRSRVEQEVRDFYSNHQAIDLIVMRKIARQKTNEDNNNKDCSVRAVLQKVSEPIAYEDSFEYEEYIPAGGSPLAHHWTEMTPSFSYLEDEFFGCADSVGTNGPPNGASFLAVGHPLVPVTRQLVGVDRFGAGGRDATQGESGNFDKMFAKEMRRRGGRMRKMALTPLEKQEWYIDEKLVKSEAAKVDLMNELSRFELKDFD;> MRHTIPFFRRSAFVPAPGSSLLNPRSQRAKVRRMVAAQKAQGENFERQALYAELGGSPSARAPRSKGERSKEATRRVGCEVAERAKHMTDAEWEGVPVDEKHAFAKYMHKVLQEHPTETTEQQRRRYFETTMADVFELDPRKTVRDEYERVKLGLPVHLKNPQYSLGVSQAVYDAADASLFDPENVHRLENAMTHVKQVFADYVHKKREGVSTEAERRMLANLTAELNLETQKHLANMFKYAEMRLRQVKLEERHHQLAEIERLRRMAQQRGGVKGRKGGSRKMSRMERLKRVINRAVGLDIAVAETVLTEMQAQEEFLQFCEVFARLTLGSGFKHTGKDENLSAYIESLRKLYSMDAATLSTLDVVQYYSSKEGAHPVDWAKRWYERALLLPLQSTPEYQKLLQIQQRDESTVKHIKETAGTGHAFACEAEAEVARIKTQKVVNLVEKMFMDPKDKRLESLHEKRLRYLAHMQMERQIRCVRENAKLFDGVENMPEAAQCRELYEKIMEKKTAQCNMTSPPEGEGSAIQSAKTEGDHCEVGPGMFNVYDDAEASSLFEKIREITLRVIRDRRVQSAAATKARMLNRIIRSLKGGERSIAEELRALHQQRKEKMTMRILGIIENDVKTEMEWLQNMEEAERPPLLPIPENMSYVSAADVQAWRELREDDERKAANPFERRRRTFQPELLGQAWSVPNKPLLFWGTGVSAVQQALRHVAEDAERKRQGLLLAPPYPCAENPWGWRLAKDILDDNN;> MYKKALHSFFLKVHPDFFHHNRSQQTVNESSVARLNELLSWAKAFKSGHLQPPPSSSFTLTFYRKPDDNMGNGETRREGSGSPVSSLVGRSMGDGSLSPTIIQSTFELPSNFAPSDNHRGTVERAVNKFLRDLLRRAACIDSVTESISEAEDATAARAEAKPLRRRPRGSQHRGAPTGPKSLLDEAVESMTVQWSLTPAPTLQELIEADQILFSRDLSPLQSAAALSTLQRHLGELNYSAWESMPVIVSNQFSIGDLTGTITIPWDFTPEQFHSFMAHNEKGVARCREVAIQYASTIEQLIAELCTALELDDILVSCSHQDALRLMELLHRNRELLIQYGLSKLTLEVGNRHATRANGVVIINCSLTSEQLRPWLKAISPKLPLQQRLYELSKQMLESTLWHLKEFRTMVEPGGVDAFSNDCTYAERLQWSKELFRIGPSLAPWDWSEMTFVLSPDVDIDWANGLLALPYNFDGDALVRYVEEVQQEAKSRKREELLAASAMQREEEERRRKQQHDEELMVECQEKGERSGDDSPTVAERMRHLYRQTNPHMDEYLASSNSRVDTLPVERPLSHAVTFNSDAEAEDQLKWEGFYAEPYVDQAPTSDIDDMAHTFMLTNRWHREEAAKKMLDQLRGTYGKKSRRFEYQKMGDVLEINNAKVQPKGFPTLTRGIKPGC;> MLSHAVPRLRLAAAAVKAAEWYAAENRRKQKGGDVIREKVDCTAPLWFDDTEQNLLAREQHVRSPAYRELHRPALTNAAMGLYGGEPGFEKAHRVWVDPDRPHIKHIYNQTALARNLRYARYGYFKRDMHLLDVDKLVRHARLLPTPGRLLTDFLYQRVPLPDKSCAALIRYQRQQIEMLEVWGRHASFQCAVEMFERMIVTNIPPVEVGVETHGEMVLCAAACGKWEEGWNVYANRARELEKESPESFILNTFFFDALLTLCVAAGRVSEGIDTLEEVIKRNLRPRGTMLNKAMILYSILGEQMSKHEASRATSEGERSYLCEPEEVEKMGLEVWSLFDFYQLPRTTASIEAYMRMCCAFNKPTLVLKAQGFADASDIRLSIECFHWLVYAIRGVAGFGDYVMDVLSQLRPRGLTPDFVLFTLSFMYCALQRDGELALAIFDQHFVHQNMNPTPEMVLLFIQACSNCEEPTAVMLERSETLIKRLEAVGSSVDLISPIYDQFLELCAHLGAVASGFSALKRIVGFGKPLTTRMINSLLLANSNAISSNGSLSMTEELVGFFTLLKIRPNADTEICVNLCRDAFGESPVVNDFIKVIGESLQGDSEKGEAPQYDEDIPVIQVPPHELRQLRTEWKLSPRDIVLRRFGQHTKPPGKAALDVGSMRGSVIPFGRSPGEQLV;> MMHRTAARLRMPRKPTPYVRKFLEGCPLPETLVDDIAGANLKSMAPFFTTAPRYIVAAESRLSKLFFHHALYPAGGARRPCRVLIVRGGRSVREPSFTINTGGGRGEVGGGSRGYRDPARRAYFYARPSTVGPFYSGNGGVSSNVAKCHSGVGSEGAGLVKRASVDGLLSPLCGVIEAHFAVGGTCNDAVATEGDGTESLTKGGEKLCVTLAGLLSGGHGGLMMDDGNCASNVRAAKRVARLLHDAAHHLSSFFYVHTQLPDSALFVSRPEASIASDGKGDGLLPSHLAREKDNDGRPSVEGVAVFRLAGGLEPTVHFAVGAPLSVLQRGVDGTASRGEKNSAEEGLNSAASTTVLPFGHIQCLLRVRTRGGKHCAAGKEGSEGTSNTPWCNTAGNDDITSNFAASGPQIAGGIVEPWKLGVSLDPKVPFFMRTLTEKRPSFSCGEGYLGTCSRSGDVDGNTVNDVSSSSGGSRTRAPGEVHMNHLLVRNDCETYLLPQRELLLSFHVPEEAEAMCKEQNEERMRRQAALGYGSPSHVFAEGPRTFARVLHGMKANLAAVEEASSTFRQGAAEGISPQVNGGSTTSGSSRVYEVRALPGDVVFVPRGWKYSVERIVGTAIIDAVAASTASPREALRAVFRTAPDPPLPQDVVRCDEGHAGAGEMPGGDSSNAEIVGVEVDAFVLCYKPYPVLSNAQASTYVAANYVHSGIDDFYAKGGNDVYHKYT;> MTGPTRALFLSSGINLGRLRLAEQFSSMNGWQSKEDPAFDAYVKERRRKENYEAFDQRVERGYAAAAKLHKAEIQNAVKRRLKSSGAKFTAETLREMSSAVTERLAWLRDVWAQIDADYRSGDSARQETAAQEISAALRGEPNDYMRWVYETKRELRFAGPVGRRAIQEELQAAELPEVLDEEVNRYHDLKLNMMEIEREVKAKYGVAGQQHWAELQAAKDEEYIQKLDEAAEVYKQLLDQSARLDESRRSELQRSYVERVHQAQVRFKAAMELEGQREQLIEAHQAMKEERMRTEREKRRQLLREAAELRAQGKKSADVLTALKERQLDANAKRQAEYELKECEDILKRKSEMLDMIAHFKHDVEEREGREMLQRQKSDEERQVNVFGFYEEVGVEDGLSISSEGTTSQGGSSGLGTVSTSTSCAKSADSNSSAQPSQKLRKEELWKVINADTYEDPFRTVHQARLDAVKTYDPAYARTFPLNLVLGRKYSRQGAGEMAAGNETDKQILQKGNNILYSFQWGLNNGTVHDLDADGGTDYFMDGAFHVRDKETGDIDWRYEKKRGGPVFRGPKFYRLGAQREAADPGERAMDPTPYTSTPREHKWRSS;> MPSASSGYTFADFLRRLERSPDSHMAPLYHEHRELFVRRHDMFARVISSVTWSKGVALVAAAGYTQAVNVTIYRALLARMLLHNRHVRQCGAGSVVPWSAALRTYSEAIATHGNAVPTRMTLSALRLCTPARQWVAAISLLMLSQANDKLTLPMLIDAAGCCATPAAWEKAMALLGRFHAQSLQVLPDSIQSLRPVGTSASTVDAAAHALLPRSEGPTPEQKHILTVINKVVSAVPWQVALSNEMCRSYLTHLVASTTLRPTEKTASLTTAVQQLPWEAFVTLMKTVTATVQEGSQGVLGSRSTPQLPPPQDGMERGDVAKSLLSNSIIREGVNLLQSEPETAIPFITTILYKLPSAEAAALFLSEATSAYRNSSSAVVAAAIRHPVVVGALLKRCADSNSWYLAASIFKSTSPTAIPCDVASDLVIQMRRANQAPLVVDVLQKYIVPSRTKLTEEAIEAALLCVLVHNRALAKASAVVAGTSPDNRTGKPNGIGVANGVHWISALSWATDLLEEGVESRILQTGTTPSVGGVNHEDPTVLLRKKTLSPRILSLLIYICVNAGSPRGGLFALGYARTVSKTELELSEEITALLYCMMYDRPREAESIIQHAVKKHGEYKGKYLGRLLVASQEAKGSALRNQT;>[2x]MRRLSVSFLPFHLIVTTQRRQFGGNSKDGHKGEDKPIERVGEVPPTGPHPFNITSGAEGQISNQQRKAHDAITQLFRDDAQRKALYQKPGRTIGAQTTTAAISTPPNEDEFEGLQPISGDAEPSSITAVEAVEQELLDDAFLYFPPAQQSASGSVATTATNELYVPGQQIIPPGLTRYRVDVQYQGNDFDGWWKSTTRQLFRREVGLDGSITRVPVAEPGTIGNAAGASRGETMGSRYHARTVLEEALAVALDVNTVRVVAGVIPEVGVSVRRLCCHVDVPSHIELQPRTVIQRATMWMEKRQQPLAILSYRRCKNQDFHARHSGLRRVYVYRILNRVAPPLFDAGLQWHVDRHLDVDRMKRFAKALEGTKDFGYFADPKMANALRRAAMSPGGFSTGAVTEENFQPKATGESHRVTRGKAPKVTMEKGPSNLDRAAALPTFNEYGQRVVQPGAHGKEYYRVATNLPTVRTVDRLDVVRQDDEVLIWFVGRSFLRHQIRNMVSVLKAAGHGLWNDLELQQALQSGFEPSRHRFKRERFPTAPAYGLTLWDVEYPDQHRDDYVQFVDSGPYEQVNIARDI;> MLIRRLRRPHSTVRGCRISSASNSDSAGAFSANGTQLPDPPYYLPHSPRFDAERCGTFNKKWLLNLPALKPLVRNSTYLPKKEELWRAPTHEALETIIGHLPYHDALRYITEHSLFLLFPTVLRARDAPLPHVIYEDFMKSCTFASLQNPPEEQFALPSVLLRTLLCMAAYHCTLDADYFTTCQMLFGRMEQQQQTTPEVLSAWVYCCTASGRVDEALTYAKYMADCSAPFDVTVFSLMQHPSLNPIEVEDGSVPHSAKGLLLQRRLGNRLHTAYRSDAVAAHGMFVYYALTLSHVRKWEVIRAAAALGVTLAERTVVLAVEVFAREKGMRCGPKTVKALTHFLAQDGTVGHLLYVLLRARKNELLPEFRDLPHTTFSEEEQELVLQCVAQRARHDDSFAVAATLVSSLVREDDPSELLMAFARAARNHHSADVCGGDGDGSVCADVPAPVPESPPSNSSEIIEKDRWAVVQASVRSLLLDVNALDQASRRDAYHKHWKNGNKGVKNKENVLAKTLTLPHDSMHTATIQRKEKELWELMRSDTPVGVRELAQLNIMEELQEAKRLERAEMAWVNPDGTF;> MKRYRSSVVTRLVRAITLRPDATVDPERYPLGYVPLDGSESVDSVWSLVKSGAFVAPLSKIETIHRAHVGIRYLTQSEYPALSSIDVVGLQTRLKELCSRLLIRRDFWVLDDYNDPELNSSFGIQNMYFDNFKWSQVLWRRFQQYVEEYFPVAEHTHLTYDEYLQLLRSFSHFEQGAKLLPLLPKRYRIHPPFGVPALSRIDMEPLLLYSQWLKNFRGPLKLDAALVIRSGCGAAVFATKLNGVPIVRGVDPNPRAVMSCRKDAQRMGRRFDSISFRVGEMFPDKDDGNGVPNSRKYDIIVFYPDQGCYNLFFTNAIGEYAPVLTGFAGTLEHFFEEAGDYLSDSGVIVLCCTNVYSILKPTEPHPIEYEIKVNRRWVLLDYYDMPVRGKGTLSHTPTDHHYRIPMEMRKCMRSELWVLHKMTSIAHFAHIHNIPGAQPPSCVVSHWRNKAIGKLRRAVLKGQVESSGGDWDDYKKRLVHLLQEQSENDEDDKAQAIRMAMDPNYPKELADRARAAIEKNMDTDKAFHNNVAKAFGDISPRERFDAYLSCYRL;> MKRIVVPHRWSEMNRVEHPPLMMKQLFQGVCGGLRWLETKSLAQYLAVRAIEEGYPSTPGVRKALHVKRAPLQKRRVVQRSTKSATAACSLPTTAAPAQLPLTSSGDALTVTGGLSLQVTKQKRLVSYDVLDCTLGSGYHAGAVLENGGPYTRVVALDCDHDAMHAARDLVEEFGGDRFRFYCCKMSEAKAMFGERSFDAIMIDGGVSDTQLEDPERGFLLDDEGGHRLDMRFGPQMGVGALEYLNTVSQHTLVSSLLAYGLLEYGQAMKMSRAITRRKPFVDSREVLTCIEQAGDELPEGGWRSQGSRRKSPMSWKFLTSLRCIINNEMYELRQGIENALLMLRDDGRLVVFSRLPWEERLVRGTVDDHPHALLSYVEDISIDDVQIYGFTRHAKMWVITRAASSAYALKNTTTLTEEKFRESSVRWLTGMYAGQTHGFPANNFTFENFERKEWVTLRRNGKPPPVDVGLDDK;> MRWSAVLCKVSKVPTRSVIPADALRYHPRYSVPRKMVLSNTFNVVGENNRYTSLKLILEKLSGHVGRRQYKMLCNLEKHYDKLKDEGIDWHELKWLSREELIVLFDKVLHLTRTERAALLPAIEAKVCGVLRQTDSRHSTVVCMNRGNANHGWRCGRNGHTNDVYFEGKAKANTAALQLCRRSSVRSVERSGVLVEVRSEPDFSVVGRFDHSLSPRVWSTPENPTFQVTTIGYEFRVHQEDPRVIPQIVEAAEEWELHANITKQVIWEMLEMYAVERDRQPLDLKPGEMGDPDIPSRHATAFNVQVVPPLSEGDEAIQVVEQRIVRADGSEVPWFQEPPPQLFSGGIPVILPFAPSIIVKSTFRQVTRSSAQDVTRQLLQPVVDVTCFLHPNVCFWWNAEDEQRCLGHIVDYAKRIPFALPFNLYFRVNLSKDLRGVQNYTEELGKRMSMKAHYFNLRSYGVR;> MLVCCRSSLSLLARATMPLCCSRRFLTHQNNIDDISGPVDTNSNSVSDGRLHCSTGEGGKASTCERVSLRTIAESLGAAAAAELRAEVERDTRDGVAAIPPLPPLGWRVRHPSGSNYFVMTRTLKNGVQSAELNNRRYRSVHDIFLQSLQKGGHKYAQKGKGSEGRQKDAKEEEEPPSQEDGKSSPKVTVGYDREGRGHRATLQRMDELHDSPKLSRADVHLTVFAPFRVYDPSLHDPTVDICEWSSFDLVVQKTVPDNMVANKLLQPLSCTPQDGALSMYVCLASVNSEMRIRSIQLLSMKEAQALVEHACFGNGEPLFLELLRRRGRRRPLVERRFDDPRLRYEEVAQPQQVADEAAVACSSSCYGPYYPAFEMLMDSCGSAGEYSRALCYGGPYVSELSRELCDALLDYIKGDLGVSDQLCEYVCQMQFFLEQEEYMTWLGQVQHVANAVSRTA;> MQRTLRSAARRKWGQKTWSPTATNGGAAPANGVSAQEALQIAYRPMPPSQTVEYEEDFGHNLMIHREYISKRCRDRVSFELSALSYSNLELRRGQEHLAGIMNRERRGVSVGASGAPDDQVQMQTDVDANSREVLSARYLFNERRLQFCDRFQNFFQSKLENSAASDSNGHEKQHLFSLMEACAVIFGCETEAARETYYRMFLGLDSETLLEEDEALRNRIADAKLVQRVLENNKGRQEVTQSPKLQQQQDQGKPLHAVSSGTSLLNDCEEERFISSIPELSLFEDETEARANGFVEGEDDVKANNGDLTAGSFSSPASSVNLPEEFEEYAPLYKAYITHAVGKGPVASYDISTLGSTGLTAERRRWRTLMEKIVREDYHTMTEVEQMDAIVLNEQLHTVKFFDLKIGDAIRDILQLLQRETGVGSSVNRDTPVGISPNNPERRV;> MLCHNRLLLVNKQTQKYRTKLRYRFRQPSVVPLRQTLQQRHNTILEVLRRRRINSGDQSPYRYVEERLYSKPSRLDREGVKVNKTYALQGLGDLEPLRYGANFGISEKDALKYETVAEKAKYMEPPIPYSSLAARKLAAGALWPAAPDPEGMISKEVRLLRHESSMSPSARAFSERVAYHLRRSLKACPGHIAEHIDFTQLIIQEVLGSRRSKEIYIVWFTVDPGARFELEPRLHQLNHWVQQLIIKRVKRRPHIPRVTWIYDGGRLERELPRDVKQELQSFVADAATTLESRVKYLKELDTMNQRMKDIPWFMPYLWSKEEKAARQKSMLADLEEVERRKNEHSSGRSAPPRTSPPPQFVR;> MHSSLIILRHAYFSALHPARRVVPGSLLPVRTQFYTRHFTSTAGPTCGDGGETYKSEPTKVGASVEGTNSGNGVTDSPSLFSSSAPTVRRRALPPSDFPENALLKCIEKEIEDEALRLDKEECPPPPPTGWEMYHAPGTSVFYGRRWWLPATASAETRATPERHTIRVQLTKRDPSLDPECDVRGEHFPFSFFVQRAPSKGEAVRRDGTFRMGDSAAAGDVKGRTEGKEEEEEEEELGLYDQSIEVRADFVDGELLVDNVVFHGTFKTGSSCSKRSGNTSPEAAAATAAGQHDNTTGGRGKVEEVRYNNIFNGYPGPNLDEAEEEVLDGLQAWLAERCVDDQFGEFVGQYSVWVEQQEYEMWLKRLRDFVAA;> MRHFRLNRCSYTPNLTSLTNQVNRSERLRKWGSAGVPPGVPRIPRLEAKGIAILHESPKVILAGRSRCNNFDSNQYMLINKATKRCLLVDASDDWPDDWAAFIGASDLTLTHVFLTHCHIDNIINLNAFLTICGSRQKQRVQVDSQDNDNREDDNGSDEIGVMWCPAEECWVQNFKRSCERYGRFEEMHQVLPMMCRSLYTPQHLVDPVIAGFSRRNARHLRRNDVLLSAATNRATSFIDFGNGVLLYYIFSPGHSPGHMMLHIPTERILFSGDLLFFNKVGRVDLPWATGVRLAESLRLLEALPDNTVVVPGHGRMTTLGRERRENKALQQCYQRQEIGKQEVSVGFNEGYL;>[2x]MSAIKRSLNVGVVGMGNMGVPIARNLGFKARSAMYLQIHSRALSKAKRVCDDLSVDGATCAMRIHDRYSTMTKWCDVIVLALADVKASRHALLEDNESLIMNARKGQIIVDHTTVDAETSRECAHEAARRGAYFLDAPMSGSPRACFNGQLLLMVGGDAETFQKMLPIFHMYADNVFHMGESGSGTAAKMISQALVASHNAAAAEALSMAHALGIEDQSKLVQVLDASWGSSTMLRRNAPLLQDLIRNPDKTPPTSAVSVDRLLSDLAHLDASLPKRGGEDEPFPVFDAALRSLAAASDAGMGDRDLASVVHYIEAGEAELRNRTHVPLGGEHLTGRTAATAANSSVNETPSTVNGSSEVPNEFGVEDFY;> MTDPVRRDPTEFLRVLRRMSRTTSWQKTMLFASKGRMVGYRLTREHYNTVLFSQSLWGRALEIVRVVRAMQEDKVQPNGATYYYIVNGMGNADHGWNYDFRINRRLEKIQHWRVALEALEACEANGFDSTDTMHNSALITLVIPGFNRWQQASLLLQRMLREDRRMHPTMVKFYHDCLVRNNRPREASSLMRLAAERGVHGYEDKWEADVYKGRPLDSEVMNESEGNGLRRQASSLAFASLMLRGDQRPLPENLQALLEEETTRNIEAERSVPVPFSAGLHATEINSVFRPRVYRQLWYKWQHIANRYRPTAALKRRQLAPRDSPTGIPGFYRI;> MVAKLQHNSAPTTLNFYEKSFQQLSDVQQRQTGLLIGAAVGDAAARALDGYTAEEVAAVAAESGSLQDEDEDPVVFASVTPREHKSGLLRHHSYTFYLFSQLLRVMATSRGDFPVQYVKNEWVATARAHPDCFVREHASLLHVLCITMQLPVIYPWADDSTLREYASGFLEFLTETPAEQAVASREDVYAYTNSVLGVALRCLQSNPDPYRNAAFMAAPGTAHVFPDDLALYCPPALVGSSHSRTEELSETDSETVPLFPARLLESDVRVVRECLVVARGAASFAEGIKAAIHLGGPVCQRSLIVGALLGARMGVRRIPISWLSATYDHVPLVTLALQVAQWSWNPPHH;>[5x]MRFINQAASDRAVINAGGRRFETLFSTLHRYPDTPFAQLFPLPGRGARQHRGREFFLDVTPHVFEYILGFLRTNQLNLPAENLQIRAEVVYSMNQWGLLEHAFPPEVIEDGEGCSTGGAVVKLPDVCVVQVCDHMQHDQGVKRHALTITYGADGFQLRSLIRRVRRDLERQLSSTYWQCYQTNERAAFFVTTKVANGTADLLTTSVTQQLVEHTESMGYSLASSYVTLSPDVVHTSVRMLIHNFTFRRSRRVEVEPGDGIALGEGSETIEAEPNIPTMHVGPRREPLNAAESIPPRNERAVNIWTVD;> MMKRTILQRCIQNKSLEIARISRSDINSRAHLPFNFDVCYELGSREFTLFSSVGSTSVLVFCNVSSRRLRSVKGGQGETEFPPKRLNVKRRRQSGSADRSPVVFSAFVSMPTSGLTIEALCCSSLGLLVVDGVSFHQGPLTESMIPQDAHPGPEGHYQGPLLNQRSLAEMVVNTRGCITSVDPFRQQESFFDGHVNPWNARSLRFGHVPVHTAKPGFSDALCHFLEVFGVNDELAFFVEDFAHLVHREEETAWTNVLKTMMGGR;> MSTSSRGILIAGLTNRARTQMAEGILRRLTAGTIFIKSGGVHHESTIHPLAVKVMKDIGIDISKQSVTSLEAARRQQNTYDVYISIDCSYERRTLDKSQPPRAEVRRRESFTVEYGDDGSGPRGGDDPVRYDPLLVPRTPSHWSVGVDATDVRRRWQIWSPRDPSIFHETSTRKFQDHLYEGEPLFMQLRQCPWRTQAKVSERWEMDEVAIRYPVERHSAHELRFVQAREQLLQRSFDLLTKLEKHYGERLLLDRALLEEFIS;> MHPRLSGQGVFPRYGGGWMHQFGHVYALQQELLNAEANNWFRAMELWHTARHEGVAMNVSHYTNILRQCVPPTAWEASLMVLKQMRRENIRPDVVGVGCALAACADANRSEEVEKVFSCFSGKLKLDSICYLALIKAKMSRGGYAEALAVGREQDADGVPFLPHTYTHLLEAAEVADDGEMALELARRMSSEQWPVSDRGREALKKLSTRHHWEEVAEYKQFVAVEDHKLSLPPTLPRG;> MWRLSRSLRSNSLHNPGPFLDGALQLIKLHLAHKNAAADKNTKACSDIEGEFLRELEAFRACFTMSSSLKVAKLYTKKLHGALSYFQLYDDPLMRQLDMIIGKQTMQPSAGRQHGVFKAPVAARLDPFFLDEREETVLPSELPNPPKPDPSTPLRERALKVPAQHRGHWVLRDPDIAITREERRTDPW;> MRRKTTLNIGQVICFSSWNDGSEGYEWKSRALSEKRSLALEFLGNVNKRVSIHDAIRLKADINKKAISNVSCPSFFSGIEGADEDEDQSDMSLCSLLGVLEGEIETDCITHLSPSDASLLKEEFLCDYDPSDTKRMAKWVNLRSETSDYQSYGAIPEGERSLWSAWYLRNIKAGKKPI;> MPPNSATRWLPFVSSDLKDYLNRYWAVMFTVGARPIETGHIRHYVSWYCTRMKVVLLDHHVYVEPLRQQLQEASRTPELPLLFVNKKLVGTLRDVELLEREKKLKDVLHFGFEWRVGGSVAATNGQKSLMGALPAPYGDAEFFRGRYRGPPVARPVVSLPTLHPFALRSEE;> MNCSSTLACHAVVSAPSTASLITSCWTPQQHCYRQLMKSLRAAYFHDRSKLFWSRHRVLVEFYKYSEEANEEAVKQLVAIGLEVAAFIDHHMRTDVERIVKHNETMMALPVAQAKKFRSDYLLAEKQHDSWCKQKIKNIMKRRPPPPYPFF;> MQRSQLARKFATQVGAYSLLRGRCHAVSTWKVMATQAVTIPMYLPVRFHSEGHAAGEEAGRTGQYLLNKDDVLTRVLEVVKNFEKVDASKVTPQSHFVNDLGLNSLDVVEVVFAIEQEFILDIPDHDAEKIQSITDAVEYISQNPMAK;> MRHFGPSIAHFPLSANQLRFKASHIRIANRKRVEMFVAKRFHLPTRLATAAPDIAAEWHDELNPMHMYPAIIGIGHVQPVWWKCAICSHSYQMSVEKRVVRGGGCPQCVVNGKRAVADGALEGEMDSQLRPKRPVMFNMRTKY;> MSRSTVFGPGSLYSFTKFGSFNRSPTNCTLNKRMKDIFRLENQKHIRNDFDRERRYRMCTKCGITTVTINFNNVPSARVGLWGRCADDKDYTHHRMVDITQREYEVLRESPVEKRLNWWRYER>MAKLIAESGSTKTEWSLVEGEHLIQRVFTEGLNPFFQTRREISRSIRLGLPDSFFKRKLEQVFFYGAGCTSAEKKSVVEASLVAQFKTPAYVESDLLAAARGLFQHDSGIACILGTGSNSCFYDGHVIVKNVRAGGYILGDEGSGAALGKQFLSDVLKKLAPQVLIDDFFEKYDLTPHDVMDVVYNRPFPNRFLAEQSCFLADYLRLDYVKGLLLSNLRSFFLRNVMQYDYLNYPIRFVGSVAYNYADLLHQVGKEFGVELSVVEETPMGGLIKYHA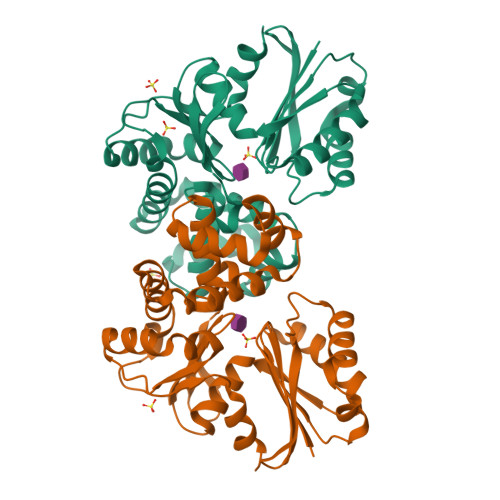FPPDDPESLEHHHHHH[6x]> GFPY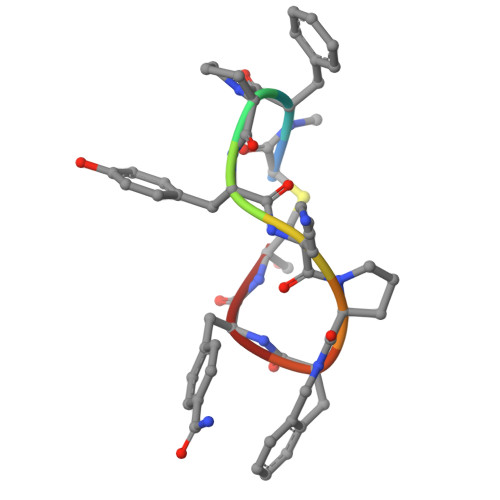KPXFC> MAGAQDFVPHTADLAELAAAAGECRGCGLYRDATQAVFGAGGRSARIMMIGEQPGDKEDLAGLPFVGPAGRLLDRALEAADIDRDALYVTNAVKHFKFTRAAGGKRRIQKTPSRTEVVACRPWLIAEMTSVEPDVVVLLGATAAKALLGNDFRVTQHRGEVLHVDDVPGDPALVATVHPSSLLRGPKEERESAFAGLVDDLRVAADV

UdgX excises uracil from uracil-containing DNA to concurrently form a covalent bond with the resulting AP-DNA. Structurally, UdgX is highly similar to family-4 UDGs (F4-UDGs). However, UdgX is unique in possessing a flexible R-loop (105KRRIH109). Our earlier studies allowed us to propose a reaction mechanism of UdgX, which involves the formation of a covalent bond between H109 of UdgX with the C1′ position of the target deoxyribose sugar concurrently with the uracil excision from this site in DNA.

Substitutions of His109 in MsmUdgX with Ser, Gly, Ala, Gln, Cys and Lys showed the loss of its covalent complex formation with DNA but gained canonical UDG activities. However, H109 substitutions by Gln or Lys, showed poor activity. Further, the overlay of all the structures of UdgX H109 mutants showed that the overall structures are very well conserved with a Cα RMSD of ca 0.2 Å. As anticipated, we note a clear difference in the sizes of the active site cavities in the various mutants. When we arranged the mutants in the order of increasing cavity sizes (left), we noted that the canonical UDG activity of the mutants increased with their increasing cavity sizes to begin with and then with a further increase in the cavity size, the UDG activity declined (right). It suggested that the initial increase in UDG activity (H109K to H109Q to H109G) occurred because of the efficiency with which the water molecule could be localized to make a nucleophilic attack on the C1′ position.> MVLRRWFPLLGVHRVGYTHPSTLPVPCAQRWDLRLARARIFQEYIEEKAPGAWQLEDERSMSPEFKTFTGYPMRD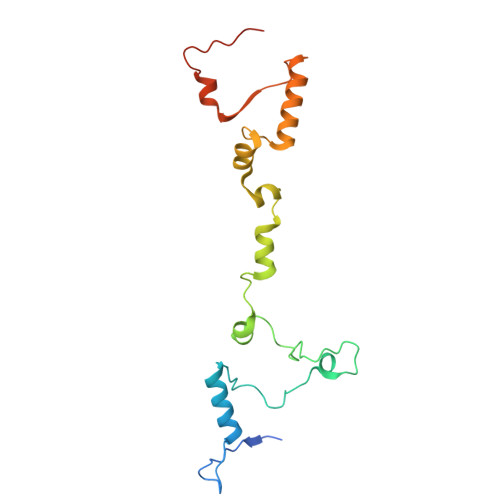MRPGYGQNLPDYIMKKRLPNNTHYELFARRDIPNEDNAMYGKYLYDMTVHGTSLPSTYRMHKDINKAQRNDRKLSGNRFKVLCSSGAKNPPSGWEPIPDATEEEED Clostridium thermocellum has extensive potential in lignocellulose biorefineries as an environmentally prominent, thermophilic, cellulolytic bacterium. Previously, five putative sugar transporters, denoted A to D and L and belonging to the ABC transport systems group, were identified in the genome of C. thermocellum, and the solute-binding lipoproteins (SBP) of these ABC transporters were shown to bind different dextrins by isothermal titration calorimetry (ITC) assays. To gain insight into the structural mechanism of the transporter specificities, 11 crystal structures, both alone and in complex with appropriate saccharides, were solved for all 5 putative sugar-binding proteins, thus providing detailed specific interactions between the proteins and the corresponding saccharides. Combined genetic, biophysical, and structural studies have provided solid evidence that transporter A and transporter B are the major glucose and cellodextrin transporters, respectively, among the five potential sugar transporters in C. thermocellum.

The crystal structures of both unliganded and glucose-liganded CbpA were determined to 2.10 and 1.85 Å resolution, respectively. Unambiguous electron density for β-d-glucose was observed in the CbpA/Glc complex, indicating that the ligand molecule was bound in a single chair conformation. Hence, the structure of unliganded CbpA assumes an open conformation, while CbpA in complex with glucose adopts a closed-conformation, resulting in approximately 37° rigid-body rotation with respect to the unliganded CbpA structure. The glucose is bound via hydrogen-bonding interactions and CH-Pi interactions with CbpA. Furthermore, the binding pocket of CbpA is distinctly small for the accommodation of a monosaccharide, and no additional space appears available for the binding of larger cellodextrins in CbpA, thus explaining the functional specificity of transporter A. However, in C. thermocellum CbpA, a phenylalanine residue (F47) occupies the corresponding location and thus cannot form a similar hydrogen bonding interaction with the substrate. In addition, W54 in CbpA adopted a conformation that is also inconsistent with hydrogen bond formation. The reduced interactions between sugar and protein in CbpA are consistent with the fact that the affinity between glucose and CbpA (KD of 240 μM) is much lower than that of the other binding proteins (KD of 1 μM or less). The ITC experiments showed that among all of the tested substrates, only CbpA binds to glucose, with a dissociation constant (KD) of 240 μM. Unlike other monosaccharide-binding proteins with strong affinities to the substrate (KD in the μM range), the binding of CbpA to glucose is remarkably weak as shown by ITC experiments.

>SAKGYVGDPSDEYYMVTFLSGIDYWKYCFEGFEDAAKAIGVTAKYTGQTDTDVSGQVAVLEQVIAQKPKGIAVTAVNSTALADTINSAIEQGISVVCFDSDSPTSNRSAYLGTGNYAAGQKAAEFLVPLVNYKGKIAVLYTVGAENSESRVQGFEDWCKQNAPEVSLVKVNDAGDTTVAADNLAAALQANDDIVGVFCVDGVAGTAGPTAVAESKKDLRVLAFDVDVTVLDKVKSGEIDGTVAQGMYNMGYWSLMMLYTEANGLSSKALPGNLDTGVVIVTKDNVDEYYPKK[4x]> VEPSGHAADRIARLPGQPAVDFDMYSGYITVDEGAGRSLFYLLQEAPEDAQPAPLVLWLNGGPGCSSVAYGASEELGAFRVKPRGAGLVLNEYRWNKVANVLFLDSPAGVGFSYTNTSSDIYTSGDNRTAHDSYAFLAKWFERF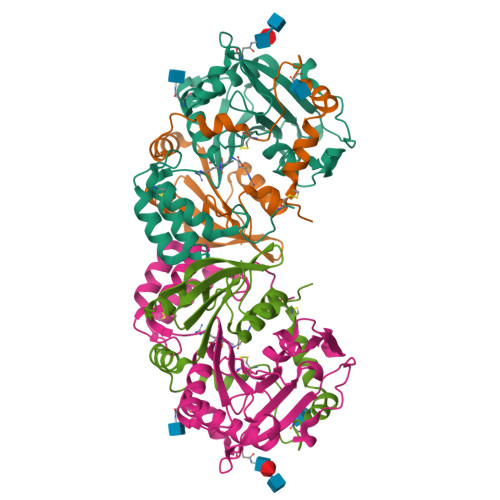PHYKYRDFYIAGESYAGHYVPELSQLVHRSKNPVINLKGFMVGNGLIDDYHDYVGTFEFWWNHGIVSDDTYRRLKEACLHDSFIHPSPACDAATDVATAEQGNIDMYSLYTPVCNITSS;> TGSYDPCTERYSTAYYNRRDVQMALHANVTGAMNYTWATCSDTINTHWHDAPRSMLPIYRELIAAGLRIWVFSGDTDAVVPLTATRYSIGALGLPTTTSWYPWYDDQEVGGWSQVYKGLTLVSVRGAGHEVPLHRPRQALVLFQYFLQGKPMPGQTKNAT;> FRVR> PRVKAAQAGR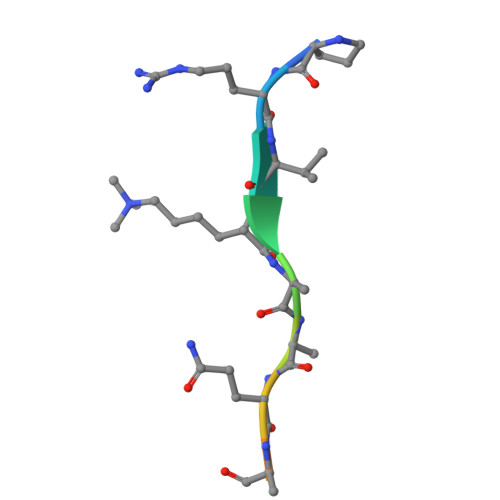QS>[4x]MSESQQLWDDVDDYFTTLLAPED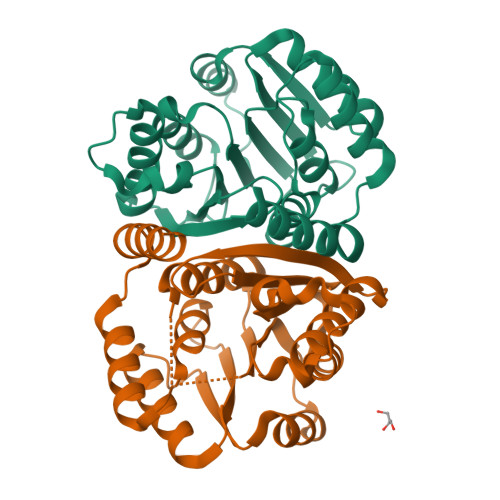EALTAALRDSDAAGLPHINVAPNQGKLLQLLAEIQGARRILEIGTLGGYSTIWLGRALPRDGRLISFEYDAKHAEVARRNLARAGLDGISEVRVGPALESLPKLADERPEPFDLVFIDADKVNNPHYVEWALKLTRPGSLIVVDNVVRGGGVTDAGSTDPSVRGTRSALELIAEHPKLSGTAVQTVGSKGYDGFALARVLPLEHHHHHH> DKRIITDDEIISLSIEFFDQNRLDRKV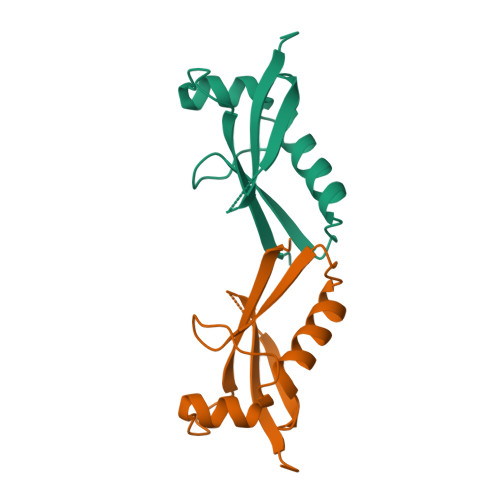NKDKEKSKEEVNDKRYLRCPAAMTVMHLRKFLRSKMDIPNTFQIDVMYEEEPLKDYYTLMDIAYIYTWRRNGPLPLKYRVRPTCKRMK> MASSHHHHHHHENLYFQGMTDTEVAQITDNPYKADFPILAANPKVAYLDSAATSQRPRVVIEAQSRFYETMNANALRGLYRWSVDATAAIEDARASIAKFIGAVDKNDKPESQQIIFTRNTSEALNLVASSLGRYALKPGDDVVISIMEHHSNIIPWQQICKATGANLVYLRMNSQYQITPEEIASKITERAKIVSVTHVSNVLGTRNDIKAIAKRTHAMGAYMVVDAAQSAPHILVNVHDLDCDLLAFSAHKMCGPMGIGVLWGRAELLNAMPPFLTGGEMIDSVTETGAVWAPVPEKFEAGTQDAAGIYATGAAIKYLNGLDMAKIEKREELLARYLVQQLCTLDFVDIVGSKLGQNHVGAVAFNVRGVHPHDVSSILDMNNVCIRAGHHCAEPLLIEL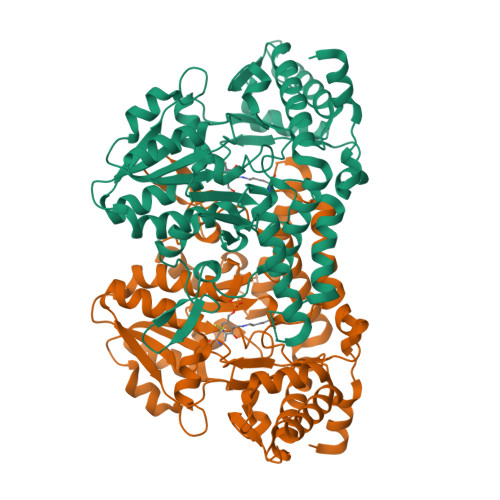HESSTCRASVAFYNDKHDIDQLIEGLNQVWKIFGSAVNTKQNKELK>[4x]SMGKLSEHLRYCDSILREMLSKKHAAYAW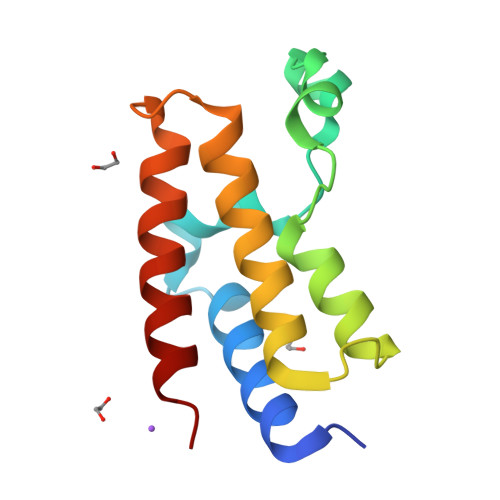PFYKPVDAEALELHDYHDIIKHPMDLSTVKRKMDGREYPDAQGFAADVRLMFSNCYKYNPPDHEVVAMARKLQDVFEMRFAKMP>[4x]MAKEEVKQKKTKEKEPDITFFHPDILEVPKDGGLPYLKGYRCKKCGQLDFKTEMCTNCWSEEFEMVPLSRRGKVYSFSDIYIGQQGLA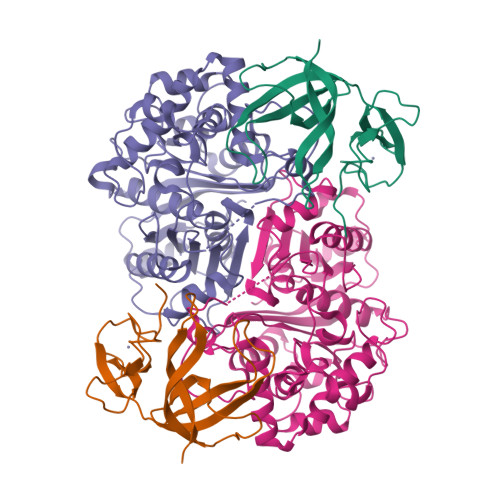TPYIFAYVDLPENLRVFAQLEGEVDTYRCDEEVELTLGPIRMNNDNLPIISYKFKKIA;>[4x]MKLQREVYIAGVGETKFGKHTVDFDVLGREAALQAMNGSNIDRPDMIQSAYVGNGMNDMTTGQAVFRGLGMCGPNLPIINVQSACSAGAMAVFCAIKDVATGVTDLSIGVGTENHTMHRQSGAAFSAARSDIETMHGAVMTGKYAMRATRYMHETGATIEDLAMITVKNRKHATHNPYAWFKGAITVEEVVNSRMVAYPMTLQQCCGIADGAAAVVVGSKEMMKKLGIAKPVKVAGVVVESGPYHNRPRDITGDDITETTSEKLYEESGIGPKEVNILELHDAFTIAELLYYECMGLCKKGDGLKFLRDGQSTYGGQCVVSPRGGLLSYGHPIGASGAAQIAQNVKQLRGECGGYQVGPTPKVAMSHVTGGGLSGTEHAACTMHMLVKGWGS> MDFSRNLYDIGEQLDSEDL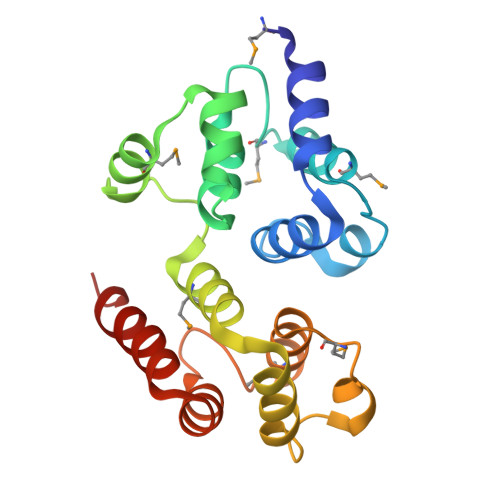ASLKFLSLDYIPQRKQEPIKDALMLFQRLQEKRMLEESNLSFLKELLFRINRLDLLITYLNTRKEEMERELQTPGRAQISAYRVMLYQISEEVSRSELRSFKGGLQEEISKCKLDDDMNLLDIFIEMEKRVILGEGKLDILKRVCAQINKSLLKIINDYEEFSKER> GSMRGSHHHHHHGSMDNSGKEAEAMALLAEAERKVKNSQSFFSGLFGGSSKIEEACEIYARAANMFKMAKNWSAAGSAFCQAAQLHLQLQSKHDAATCFVDAGNAFK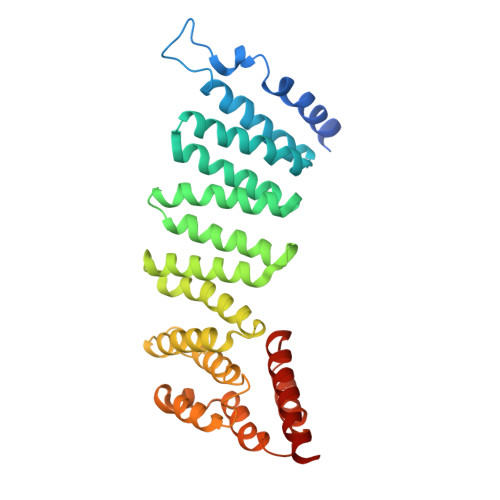KADPQEAINCLMRAIEIYTDMGRFTIAAKHHISIAEIYETELVDIEKAIAHYEQSADYYKGEESNSSANKCLLKVAGYAAQLEQYQKAIDIYEQVGTNAMDSPLLKYSAKDYFFKAALCHFCIDMLNAKLAVQKYEELFPAFSDSRECKLMKKLLEAHEEQNVDSYTEAVKEYDSISRLDQWLTTMLLRIKKTIQGDEEDLR>[2x]SEQWRE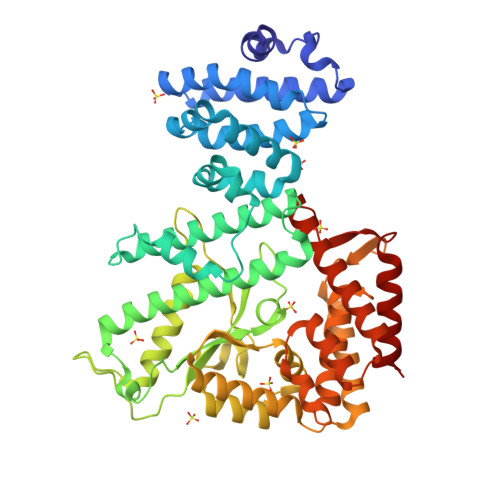LWQDALQEDDTTPVLAHLSEDDRKQVLTLIADFRKELDKRTIGPRGRQVLDHLMPHLLSDVCAREDAAVTLSRITALLVGIVTRTTYLELLSEFPAALKHLISLCAASPMIASQLARYPLLLDELLDPNTLYQPTATDAYRDELRQYLLRVPEDDEEQQLEALRQFKQAQLLRIAAADIAGTLPVMKVSDHLTWLAEAMIDAVVQQAWVQMVARYGKPNHLNEREGRGFAVVGYGKLGGWELGYSSDLDLIFLHDCPMDAMTDGEREIDGRQFYLRLAQRIMHLFSTRTSSGILYEVDARLRPSGAAGMLVTSAEAFADYQKNEAWTWEHQALVRARVVYGDPQLTAHFDAVRREIMTLPREGKTLQTEVREMREKMRAHLGNKHRDRFDIKADEGGITDIEFITQYLVLRYAHEKPKLTRWSDNVRILELLAQNDIMEEQEAMALTRAYTTLRDELHHLALQELPGHVSEDCFTAERELVRASWQKWLVEE> GSILTRWLLIPPVNARLIGRYRDYRRHGASAFSATLGCFWMILAWIFIPLEHPRWQRIRAEHKNLYPHINASRPRPLDPVRYLIQTCWLLIGASRKETPKPRRRAFSGLQNIRGRYHQWMNELPERVSHKTQHLDEKKELGHLSAGARRLILGIIVTFSLILALICVTQPFNPLAQFIFLMLLWGVALIVRRMPGRFSALMLIVLSLTVSCRYIWWRYTSTLNWDDPVSLVCGLILLFAETYAWIVLVLGYFQVVWPLNRQPVPLPKDMSLWPSVDIFVPTYNEDLNVVKNTIYASLGIDWPKDKLNIWILDDGGREEFRQFAQNVGVKYIARTTHEHAKAGNINNALKYAKGEFVSIFDCDHVPTRSFLQMTMGWFLKEKQLAMMQTP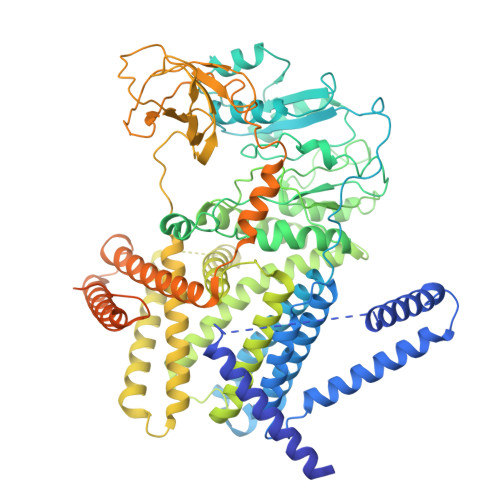HHFFSPDPFERNLGRFRKTPNEGTLFYGLVQDGNDMWDATFFCGSCAVIRRKPLDEIGGIAVETVTEDAHTSLRLHRRGYTSAYMRIPQAAGLATESLSAHIGQRIRWARGMVQIFRLDNPLTGKGLKFAQRLCYVNAMFHFLSGIPRLIFLTAPLAFLLLHAYIIYAPALMIALFVLPHMIHASLTNSKIQGKYRHSFWSEIYETVLAWYIAPPTLVALINPHKGKFNVTAKGGLVEEEYVDWVISRPYIFLVLLNLVGVAVGIWRYFYGPPTEMLTVVVSMVWVFYNLIVLGGAVAVSVESKQVRRSHRVEMTMPAAIAREDGHLFSCTVQDFSDGGLGIKINGQAQILEGQKVNLLLKRGQQEYVFPTQVARVMGNEVGLKLMPLTTQQHIDFVQCTFARADTWALWQDSYPEDKPLESLLDILKLGFRGYRHLAEFAPSSVKGIFRVLTSLVSWVVSFIPPRPERSETAQPSDQALAQQHHHHHHLEHHHHHH>MEAEQVWKLWRRVLRDERLQAQLFSATDATHWLSGFSESESKILSVYAQQFDRVKWFVENYQFRLVNSFLNALETGAPLSLRALLHINVDLNAQSKAFLRDRQWRDYGPQVYTYCEDVLGFLAEADELQGYPEILDLMRLERESVRLYRGLVDPESLPADNRYQRTSMARLYETRFALSGWLRQKDQLGLTRLPESTEHVLIYLPTLQARHKFTLINAQAARLYNCLEQPQSAAGLFMLINSDSASVPGSADLALLDRLEQLNAIRKPL[2x];>MPDFVKPAPIGVGIQYNPEILDWFPFEDIQVDILEILLDNIMAPMDGPQIIKPSAQAMIERLGQKFTLLAHSNYGCDFGFSALEETAAVQRHVPLAKMLNSPWVANHCFYGDQSWLDIWSSPIQFSAAEVARCADRAQSLQTLYGMPLAHENAAYYLECPGAEMREAEFLARLVQRSGTFLHLDLHNIYTNHLNLKGFDLKDYMDTLPLDKVISVHLAGGSWHGGLYHDWHDACVPEPVWDLYEDLLSRAQPSAVILEYQGQAHHAQTRIMDASDESMIVRDVQRAQAIWSRYNRHPQERQYGS[2x]

The next unusual PTM reaction on TglA-Cys is performed by a complex formed by TglH and TglI, in which the cysteine β-methylene (β-CH2) of TglA-Cys is removed to generate TglA-CysΔCH2. Like MbnB and MbnC, TglH and TglI of the TglHI holoenzyme likely function as a catalytic and recruitment subunit, respectively, to achieve TglA-Cys modification. Here, we report the structures of TglHI in the absence of Fe ions, with two Fe ions, and with three Fe ions (apoTglHI, TglHI-2Fe and TglHI-3Fe, respectively). The interaction with TglI is required for TglH catalytic activity, indicating that the TglHI complex acts as a holoenzyme for 3-thiaGlu generation, akin to MbnBC.

Unlike the reported homologous structure of MbnB,32,33 no extra electron density in the active center of the TglH map was observed, suggesting that the crystallized protein lacks metal ions, and therefore, this structure was termed apoTglHI. ApoTglH adopts an eight-stranded triosephosphate isomerase (TIM)-barrel fold consisting of eight β-strands wrapped around ten α-helixes and two η-helixes. TglI consists of an N-terminal helix domain (NTD), a linker loop, and a C-terminal domain (CTD) identified as an RRE domain. Two extended loops of apoTglH, L1 (residues 41–53) and L3 (residues 151–166), are inserted into two grooves formed by α7–8 (G2) and α1–3 (G1) of the TglI NTD, respectively, forming a mortise and tenon-like structure. L1 embedded in G2 thereby forms a hydrophobic interface I with a buried surface area of ~573 Å2. Moreover, L3 buried in G1 forms a hydrophobic interface II with a buried surface area of ~320 Å2. Notably, the TglI CTD is not involved in the interaction between apoTglH and TglI, likely because of the role of the CTD in recognition of the longer LP of the cognate substrate. Although apoTglH and MbnB exhibit comparable overall structures, the specific inter-subunit interactions of apoTglHI are distinct from those of MbnBC. In the closed state, two iron ions are bound in the active site (TglHI-2Fe), whereas in the open state, iron ions are absent from the active site (apoTglHI), indicating that the intrinsic flexibility of L2 and L4 allows Fe loading in TglH to result in TglHI activation.>MRSRRVDVMDVMNRLILAMDLMNRDDALRVTGEVREYIDTVKIGYPLVLSEGMDIIAEFRKRFGCRIIADFKVADIPETNEKICRATFKAGADAIIVHGFPGADSVRACLNVAEEMGREVFLLTEMSHPGAEMFIQGAADEIARMGVDLGVKNYVGPSVRPERL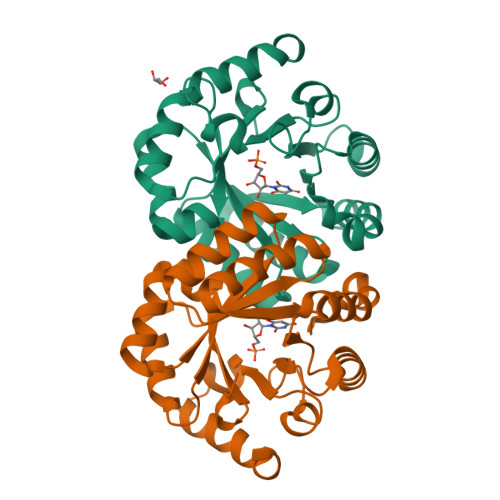SRLREIIGQDSFLISPGAGAQGGDPGETLRFADAIIVGRSIYLADNPAAAAAGIIESIKDLLNP[2x]>MRGSHHHHHHGSMDKNIIIGAMTALITPFKNGKVDEQSYARLIKRQIENGIDAVVPVGTTGESATLTHEEHRTCIEIAVETCKGTKVKVLAGAGSNATHEAVGLAKFAKEHGADGILSVAPYYNKPTQQGLYEHYKAIAQSVDIPVLLYNVPGRTGCEISTDTIIKLFRDCENIYGVKEASGNIDKCVDLLAHEPRMMLISGEDAINYPILSNGGKGVISVTSNLLPDMISALTHFALDENYKEAKKINDELYNINKILFCESNPIPIKTAMYLA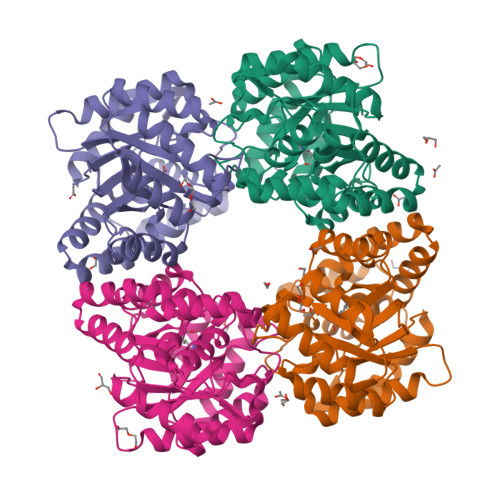GLIESLEFRLPLCSPSKENFAKIEEVMKKYKIKGF[6x]1-(5-chloro-6-fluoro-1H-benzimidazol-2-yl)-1H-pyrazole-4-carboxylic acid | C11 H6 Cl F 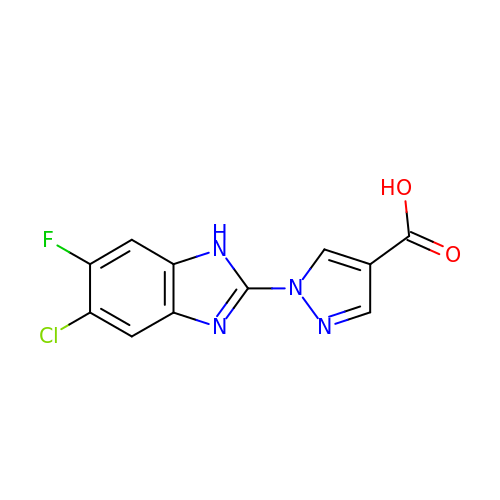N4 O2 | VOINEICHGDKMIS-UHFFFAOYSA-N The adaptor protein, speckle-type BTB/POZ protein (SPOP), recruits substrates to the cullin-3-subclass of E3 ligase for selective protein ubiquitylation. SPOP recruits substrates via its N-terminal MATH domain, whereas a central BTB domain mediates dimerization and interactions with Cul3. Here, we show that MyD88 interacts with SPOP through a long degron that contains the established SPOP-binding consensus and an N-terminal site that we name the Q-motif. We determine the structural basis of these interactions and show that the Q-motif interacts with an unexplored binding pocket on the SPOP MATH domain.

MyD88 interacts with SPOP through a sequence (134VDSSV138; MyD88 SBC) located between the death- and TIR domains. The side chain of MyD88 Val134 is buried in a hydrophobic pocket that is contributed by SPOP residues Phe102, Tyr123, Trp131, and Phe133, whereas the side chains of MyD88 residues 135DSS137 are involved in hydrogen bonding with the side chains of SPOP residues Tyr87, Lys129, and Asp130. The side chains of MyD88 Leu129 and Gln130 sit in a hydrophobic pocket that is contributed by SPOP residues Phe136, Ile137, and Phe141, with the side chain of Gln130 also forming hydrogen bonds with the backbone carbonyl groups of SPOP Lys115 and Phe136. The +5 residue of the MyD88 SBC (Val138) differs from the defined consensus. MyD88 Val138 cannot make these contacts, and instead, the backbone NH group of MyD88 Arg140 forms a hydrogen bond with the side chain of SPOP Asp77, thereby directing the C-terminus of the MyD88 peptide in a different direction from that observed in other SPOP substrates. Of note, the Cα B-factors of the C-terminal MyD88 residues, 138VPR140, were relatively high, and these residues were not modeled in a crystal structure of SPOPMATH in complex with a longer MyD88 peptide (128PLQVAAVDSSVPRTAELAG146). This suggests that the residues located C-terminal to the SBC are highly flexible, as observed in structures of other SPOP substrates.

> APKVVKFSYMWTINNFSFCREEMGEVIKSSTFSSGANDKLKWCLRVNPKGLDEESKDYLSLYLLLVSCPKSEVRAKFKFSILNAKGEETKAMESQRAYRFVQGKDWGFKKFIRRDFLLDEANGLLPDDKLTLFCEVSVVQD;> KPLQVAAVDSSVPRTAELAG>[2x]NVEEETKYIELMIVNDHLMFKKHRLSVVHTNTYAKSVVNMADLIYKDQLKTRIVLVAMETWATDNKFAISENPLITL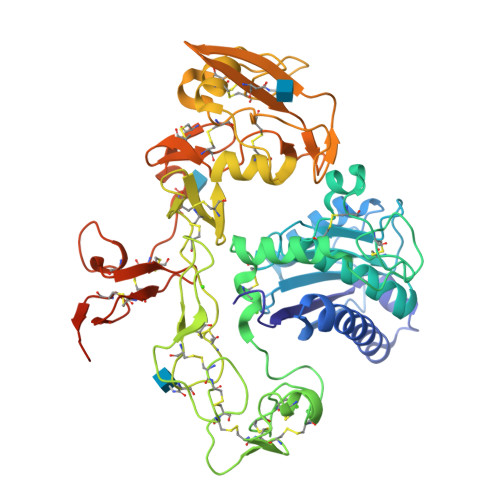REFMKYRRDFIKEKSDAVHLFSGSQFESSRSGAAYIGGICSLLKGGGVNEFGKTDLMAVTLAQSLAHNIGIISDKRKLASGECKCEDTWSGCIMGDTGYYLPKKFTQCNIEEYHDFLNSGGGACLFNKPSKLLDPPECGNGFIETGEECDCGTPAECVLEGAECCKKCTLTQDSQCSDGLCCKKCKFQPMGTVCREAVNDCDIRETCSGNSSQCAPNIHKMDGYSCDGVQGICFGGRCKTRDRQCKYIWGQKVTASDKYCYEKLNIEGTEKGNCGKDKDTWIQCNKRDVLCGYLLCTNIGNIPRLGELDGEITSTLVVQQGRTLNCSGGHVKLEEDVDLGYVEDGTPCGPQMMCLEHRCLPVASFNFSTCLSSKEGTICSGNGVCSNELKCVCNRHWIGSDCNTYFPHNDDAKTGITLSGNGVAGTNHHHHHH> MEDISTEKTVESLEAIRHRIAQIVQSLTHFLAILHQSESLSPWPTIHKNFNILLSQIHSLSNNLAAHSHT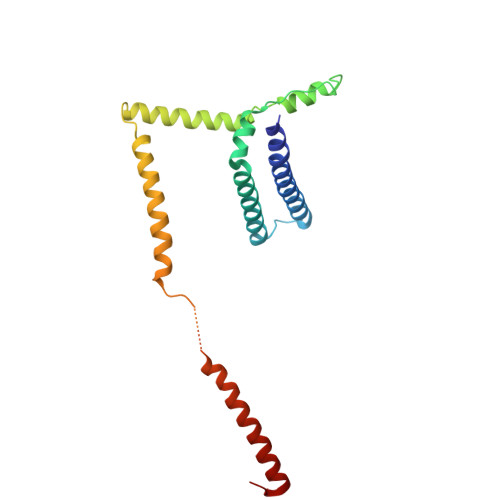LQTTSIYPSLEFPVKEQEPLLTTLLRTKALPEVEEWEANTLQEYEASISSQPKKKEANDAYQKDQLWDQARIIFMEERENYSWFDFVTRRQESEGEFVSQRQLEIDRATEEQNANQMLTDILSFMKSGKR>[4x]GAMGSMNLLIMGLPGAGKGTQAAKIVEQFHVAHISTGDMFRAAMANQTEMGVLAKSYIDKGELVPDEVTNGIVKERLSQDDIKETGFLL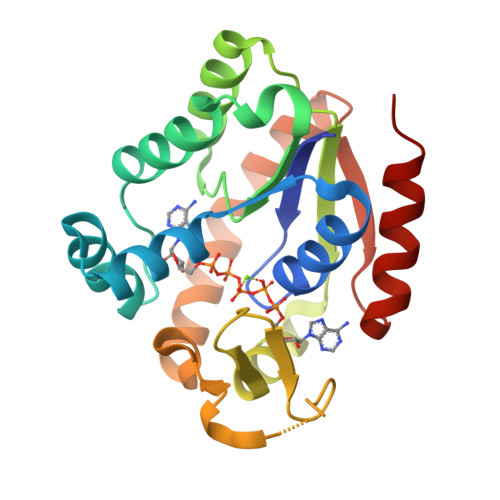DGYPRTIEQAHALDKTLAELGIELEGIINIEVNPDSLLERLSGRIIHRVTGETFHKVFNPPVDYKEEDYYQREDDKPETVKRRLDVNIAQGEPIIAHYRAKGLVHDIEGNQDINDVFSDIEKVLTNLK>AAAVQPLARDAMAYVLAGGRGSRLKELTDRRAKPAVYFGGKARIIDFALSNALNSGIRRIGVATQYKAHSLIRHLQRGWDFFRPERNESFDILAASQRVSETQWYEGTADAVYQNIDIIEPYAPEYMVILAGDHIYKMDYEYMLQQHVDSGADVTIGCLEVPRMEATGFGVMHVNEKDEIIDFIEKPADPPGIPGNEGFALASMGIYVFHTKFLMEALRRDAADPTSSRDFGKDIIPYIVEHGKAVAHRFADSCVRSDFEHEPYWRDVGTIDAYWQANIDLTDVVPD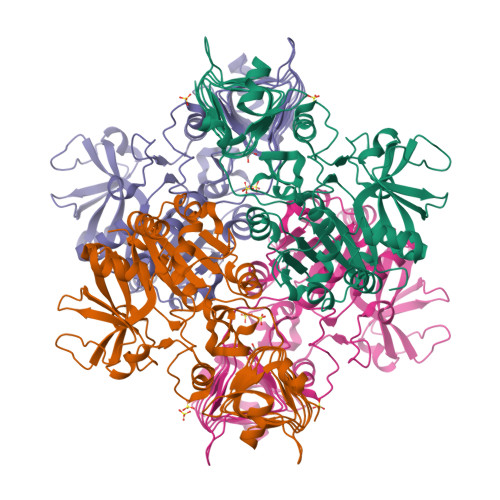LDIYDKSWPIWTYAEITPPAKFVHDDEDRRGSAVSSVVSGDCIISGAALNRSLLFTGVRANSYSRLENAVVLPSVKIGRHAQLSNVVIDHGVVIPEGLIVGEDPELDAKRFRRTESGICLITQSMIDKLDL[20x]> GHMEKLHE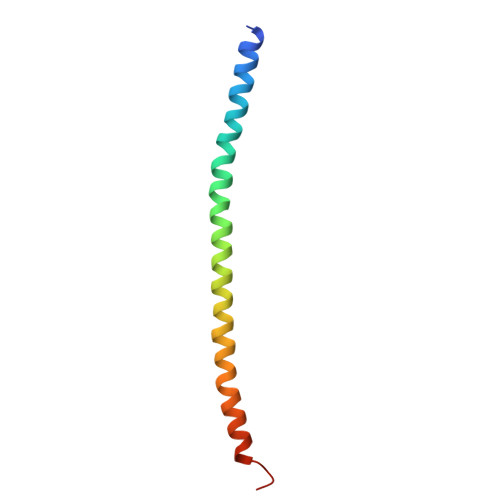ANNELQKKRAIIEDLEPRFNNSSLKIEELQEALRKKEEEMKQMEERYKKYLEKAKSVIRTLDPKQNQ>MHHHHHHLKFMLDTNICIFTIKNKPASVRERFNLNQGKMCISSVTLMELIYGAEKSQMPERNLAVIEGFVSRIDVLDYDAAAATHTGQIRAELARQGRPVGPFNQMIAGHARSRGLIIVTNN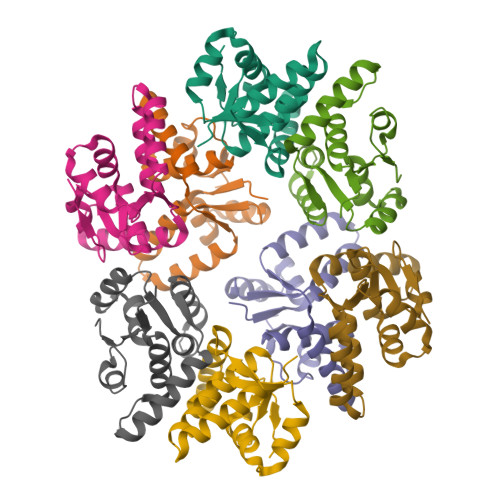TREFERVGGLRTEDWS[8x]> MAQKTFTVTADSGIHARPATTLVQAASKFDSDINLEFNGKT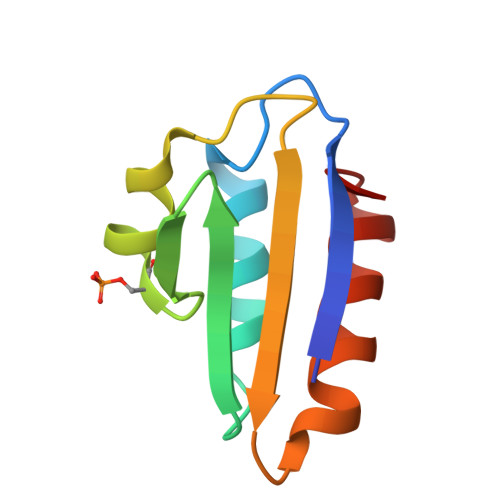VNLKSIMGVMSLGIQKGATITISAEGSDEADALAALEDTMSKEGLGE> MASSHHHHHHSSGLVPRGSHMTEATAGTVTVNAITSDDTIDGIELGQTISISGKAVGGDISVGDVVKMTINNTEYSTTVKAGGIWMIAGVLGSDLAADSEFDVVVTSSDAAGNKVQSIGTSTHSVDLSAEANFSLAEGQQHVLTNLPEGFGFPDGTTEVVTNFGGTITLGDDGEYRYDAPVRDHGDAVSDKDSVTVTLEDGRTFTVNLDIQDSAPVAVDDQDSIVVQHEEFEVSEIAASWVSYTHGESVTTFDGTSDLGGVDNDSAKDQIRWGNPAESKQSGYGFIDNDSNLEGRFDLNQDISVGTFTHYNYPVYSGGAITSAEMSVEFSVLDHLGVSTPVTLTVNFDHNETPNTNDVNASRDIVTVQNTHVTFERDGDIYTVQIVGFREVGNPDGEVVTSIYTNENAATSYELVVRVVEGDGYSLPSTEGNIFDDNGLGADSLGADGSVTVVGVAVGAIVSSNESVGHSIEGQYGNLVLNSDGSYVYDVTASVSDIPAGATESFAYLI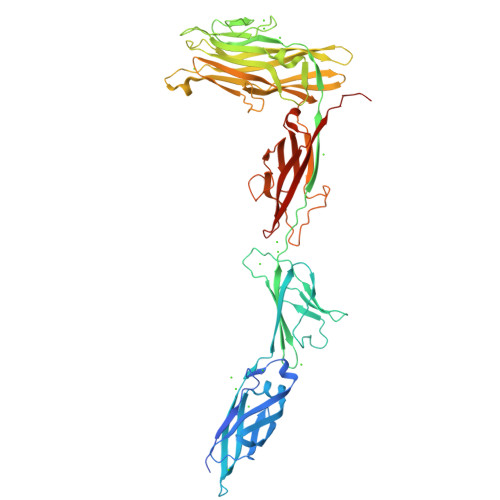QDQDGSTSSANLSINVGTNTAPKAQDDSTPD> MHHHHHHADQTNPYKLMDEAAQKTFDRLKNEQPQIRANPDYLRTIVDQEL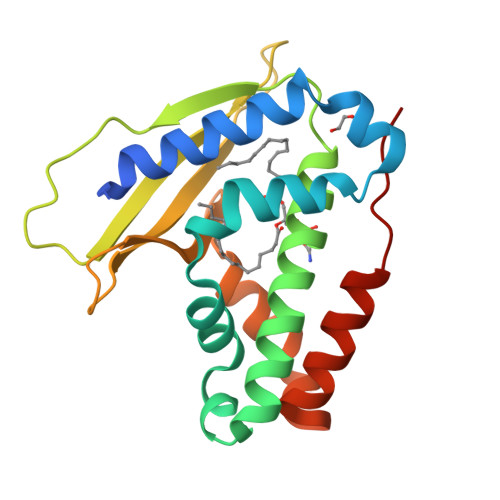LPYVQVKYAGALVLGQYYKSATPAQREAYFAAFREYLKQAYGQALAMYHGQTYQIAPEQPLGDKTIVPIRVTIIDPNGRPPVRLDFQWRKNSQTGNWQAYDMIAEGVSMITTKQNEWGTLLRTKGIDGLTAQLKSISQQKITLEEKK>GSTGSMFKLLLIFADPAEAARTLSLFPFSLNKENFYTYHTENVLLDVMVLKTWGYRGVVQALSPPPSGYDLWINAGFAGAANPNIPLLKTYTITSVKELTPTTSVEEELEVTPIPRLPLAQLTSVRSPYRDGFHEHLQLVDMEGFFIAKQASLVACPCSMIKVSS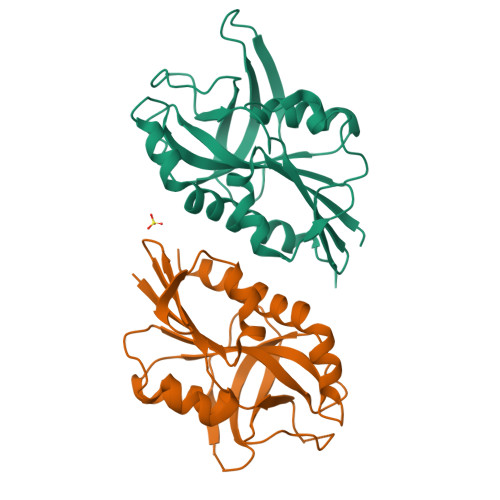NYTTREGQDFLKNNKVKLSQKLAEAIFPIYSSFIDV[2x]>[4x]MSEITLGRYLFERLKQVEVQTIFGLPGDFNLSLLDNIYEVPGMRWAGNANELNAAYAADGYARLKGMSCIITTFGVGELSALNGIAGSYAEHVGVLHVVGVPSVSSQAKQLLLHHTLGNGDFTVFHRMSSNISETTAMITDINTAPAEIDRCIRTTYV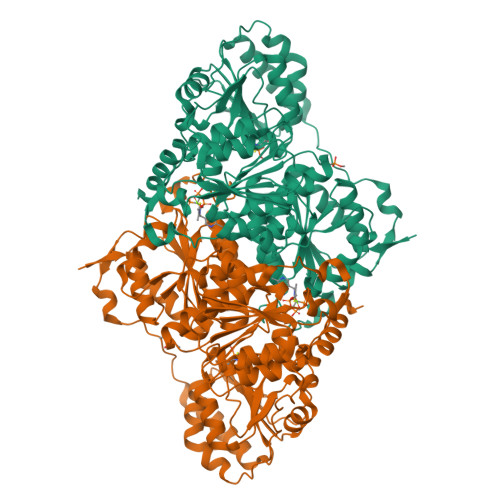SQRPVYLGLPANLVDLTVPASLLDTPIDLSLKPNDPEAEEEVIENVLQLIKEAKNPVILADACCSRHDAKAETKKLIDLTQFPAFVTPMGKGSIDEKHPRFGGVYVGTLSSPAVKEAVESADLVLSVGALLSDFNTGSFSYSYKTKNIVEFHSDYTKIRSATFPGVQMKFALQKLLTKVADAAKGYKPVPVPSEPEHNEAVADSTPLKQEWVWTQVGEFLREGDVVITETGTSAFGINQTHFPNNTYGISQVLWGSIGFTTGATLGAAFAAEEIDPKKRVILFIGDGSLQLTVQEISTMIRWGLKPYLFVLNNDGYTIERLIHGETAQYNCIQNWQHLELLPTFGAKDYEAVRVSTTGEWNKLTTDEKFQDNTRIRLIEVMLPTMDAPSNLVKQAQLTAATNAKN> MLKILWTYILFLLFISASARAEKPWYFDAIGLTETTMSLTDKNTPVVVSVVDSGVAFIGGLSDSEFAKFSFTQDGSPFPVKKSEALYIHGTAMASLIASRYGIYGVYPHALISSRRVIPDGVQDSWI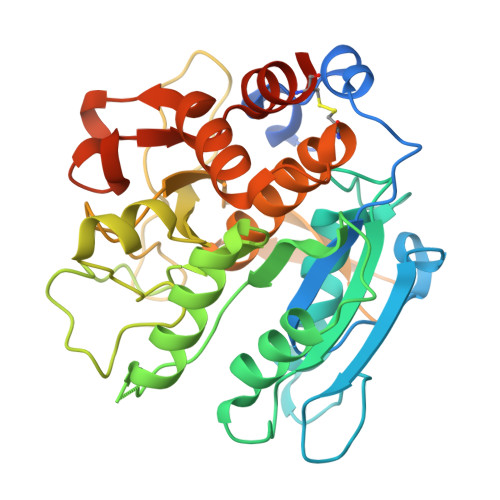RAIESIMSNVFLAPGEEKIINISGGQKGVASASVWTELLSRMGRNNDRLIVAAVGNDGADIRKLSAQQRIWPAAYHPVSSVNKKQDPVIRVAALAQYRKGETPVLHGGGITGSRFGNNWVDIAAPGQNITFLRPDAKTGTGSGTSEATAIVSGVLAAMTSCNPRATATELKRTLLESADKYPSLVDKVTEGRVLNAEKAISMFCKKNYIPVRQGRMSEEL>GASGDLYEVERIVDKRKNKKGKWEY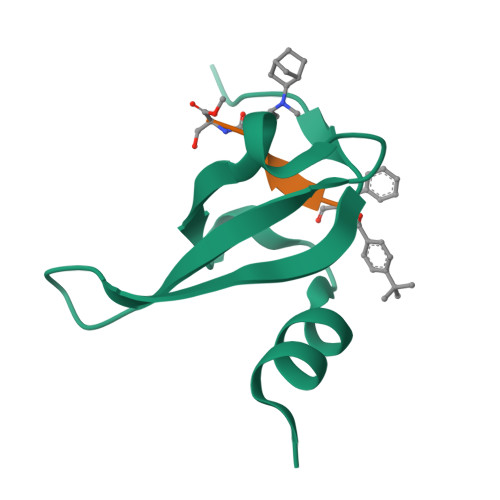LIRWKGYGSTEDTWEPEHHLLHCEEFIDEFNGLHMSK[6x]>[3x]SNAMAVDMFIKIGDVKGESKDKTHAEEIDVLAWSWGMSQSGSMHMGGGGGAGKVNVQDLSFTKYIDKSTPNLMMACSSGKHYP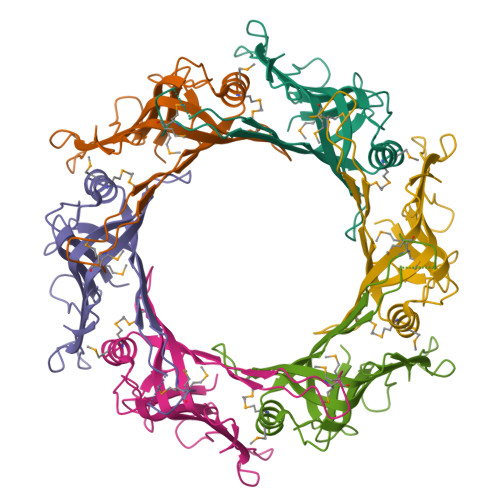QAKLTIRKAGGENQVEYLIITLKEVLVSSVSTGGSGGEDRLTENVTLNFAQVQVDYQPQKADGAKDGGPVKYGWNIRQNVQA>[4x]RTFLNLTKPLCEVNSWHILSKDNAIRIGEDAHILVTREPYLSCDPQGCRMFALSQGTTLRGRHANGTIHDRSPFRALISWEMGQAPSPYNTRVECIGWSSTSCHDGMSRMSICMSGPNNNASAVVWYGGRPITEIPSWAGNILRTQESECVCHKGVCPVVMTDGPANNRAATKIIYFKEGKIQKIEELAGNAQHI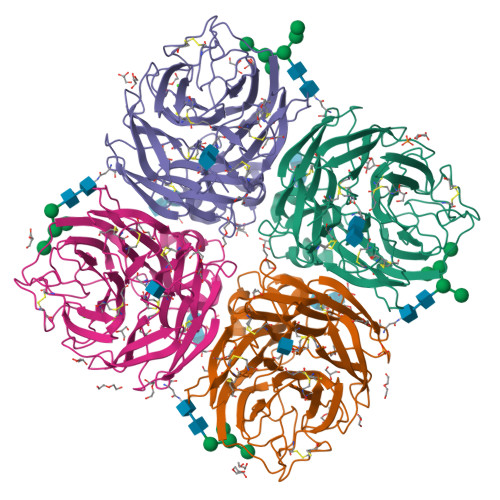EECSCYGAGGVIKCICRDNWKGANRPVITIDPEMMTHTSKYLCSKVLTDTSRPNDPTNGNCDAPITGGSPDPGVKGFAFLDGENSWLGRTISKDSRSGYEMLKVPNAETDIQSGPISNQVIVNNQNWSGYSGAFIDYWANKECFNPCFYVELIRGRPKESSVLWTSNSIVALCGSKKRLGSWSWHDGAEIIYFE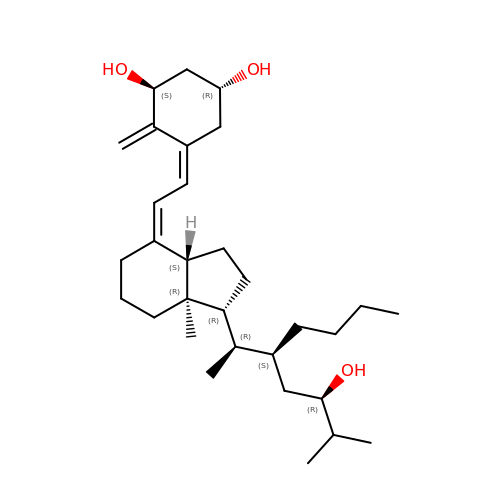(1R,3S,5Z)-5-[(2E)-2-{(1R,3aS,7aR)-1-[(1R,2S,4R)-2-butyl-4-hydroxy-1,5-dimethylhexyl]-7a-methyloctahydro-4H-inden-4-ylidene}ethylidene]-4-methylidenecyclohexane-1,3-diol | C31 H52 O3 | CJFXAKUNOBKWSJ-ZUNQKOJFSA-N>KKARMTVDKDYKIAEIDKRIYGSFVEHLGRAVYDGLYQPGNSKSDEDGFRKDVIELVKELNVPIIAYPGGNFVSNYFWEDGVGPVEDRPRRLDLAWKSIEPNQVGINEFAKWCKKVNAEIMMAVNLGTRGISDACNLLEYCNHPGGSKYSDMRIKHGVKEPHNIKVWCLGNEMDGPWQVGHKTMDEYGRIAEETARAMKMIDPSIELVACGSSSKDMPTFPQWEATVLDYAYDYVDYISLHQYYGNKENDTADFLAKSDDLDDFIRSVIATCDYIKAKKRSKKDIYLSFDEWNVWYHSNNEDANIMQNEPWRIAPPLLEDIYTFEDAL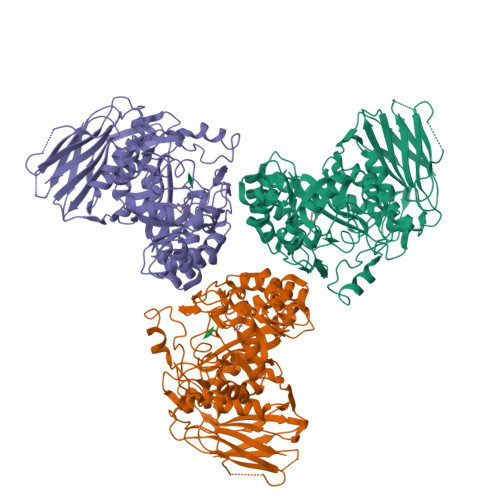LVGLMLITLMKHADRIKIACLAQLINVIAPIVTERNGGAAWRQTIFYPFMHASKYGRGIVLQPVINSPLHDTSKHEDVTDIESVAIYNEEKEEVTIFAVNRNIHEDIVLVSDVRGMKDYRLLEHIVLEHQDLKIRNSVNGEEVYPKNSDKSSFDDGILTSMLRRASWNVIRIG[6x]>[4x]MFKIGSVLKQIRQELNYHQIDLYSGIMSKSVYIKVEADSRPISVEELSKFSERLGVNFFEILNRAGMNTKSVNETGKEKLLISKIFTNPDLFDKNFQRIEPKRLTSLQYFSIYLGYISIAHHYNIEVPTFNKTITSDLKHLYDKRTTFFGIDCEIVSNLLNVLPYEEVSSIIKPMYPIVDSFGKDYDLTIQTVLKNA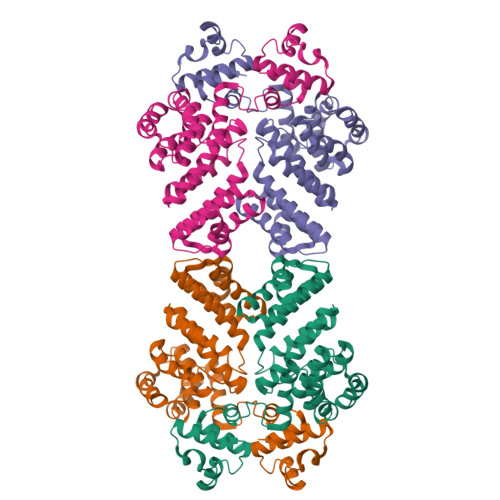LTISIMNRNLKEAQYYINQFEHLKTIKNISINGYYDLEINYLKQIYQFLTDKNIDSYLNAVNIINIFKIIGKEDIHRSLVEELTKISAKEKFTPPKEVTMYYENYVAIENNPIPEIKEQS In many Gram-positive bacteria, the redox-sensing transcriptional repressor Rex controls central carbon and energy metabolism by sensing the intra cellular balance between the reduced and oxidized forms of nicotinamide adenine dinucleotide; the NADH/NAD+ ratio. Here, we report high-resolution crystal structures and characterization of a Rex ortholog (Gbs1167) in the opportunistic pathogen, Streptococcus agalactiae, also known as group B streptococcus (GBS). Rex is a homodimer consisting of two domains, an N-terminal DNA recognition domain and a C-terminal Rossmann-like dinucleotide-binding and dimerization domain. The dimerization of Rex is stabilized by the swapping of the C-terminal α-helices and the dimer binds to a consensus Rex OPerator (ROP) sequence (TTGTGAAN4TTCACAA) to repress expression of target genes.

The Rex-NAD+ complex crystalized in two different space groups, P21 and P212121. The higher resolution P21 form contained two NAD+ molecules per Rex dimer whereas the P212121 form only contained one NAD+ molecule per dimer. The superimposition of the Rex-NAD+ complex and the DNA bound conformers revealed root-mean-square deviations (RMSD) ranging from 3.1 Å (for NAD1) to 4.0 Å (for NAD2). These changes are confined primarily to rearrangements of the N-terminal DNA binding domain. In order to bind to the ROP the DNA binding domain of one of the subunits of the Rex-NAD+ complex must rotate 26.2o. The rotation leads to an increased distance between the recognition helices (α3) from NAD1 (18 Å), NAD2 (15 Å to 34 Å). Comparisons of the three GBS Rex structures reveal significant inter-domain movement between the nucleotide binding domain and the DNA binding domain. Similar to a proposed model for B. subtilis Rex, binding NAD+ does not lock the protein in the DNA binding conformation, but rather appears to act to increase the rigidity of Rex, thereby limiting the conformational flexibility of the protein and stabilizing the interaction with DNA. The allosteric effect of DNA on NAD+ binding observed in this study of GBS Rex supports this idea.

>MIMDKSIPKATAKRLSLYYRIFKRFNTDGIEKASSKQIADALGIDSATVRRDFSYFGELGRRGFGYDVKKLMNFFAEILNDHSTTNVMLVGCGNIGRALLHYRFHDRNKMQISMAFDLDSNDLVGKTTEDGIPVYGISTINDHLIDSDIETAILTVPSTEAQEVADILVKAGIKGILSFSPVHLTLPKDIIVQYVDLTSELQTLLYFMNQQR[2x]> MGSSHHHHHHSSGLVPRGSVGGCLAKDGLQQSKCPDTTPKRRRASSLSRDAERRAYQWCREYLGGAWRRVQPEELRVYPVSG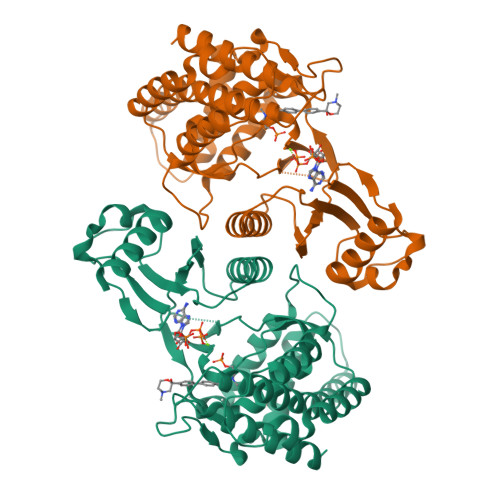GLSNLLFRCSLPDHLPSVGEEPREVLLRLYGAILQGVDSLVLESVMFAILAERSLGPQLYGVFPEGRLEQYIPSRPLKTQELREPVLSAAIATKMAQFHGMEMPFTKEPHWLFGTMERYLKQIQDLPPTGLPEMNLLEMYSLKDEMGNLRKLLESTPSPVVFCHNDIQEGNILLLSEPENADSLMLVDFEYSSYNYRGFDIGNHFCEWVYDYTHEEWPFYKARPTDYPTQEQQLHFIRHYLAEAKKGETLSQEEQRKLEEDLLVEVSRYALASHFFWGLWSILQASMSTIEFGYLDYAQSRFQFYFQQKGQLTSVHSSS> FAGGTVSQRCLSCICKMESGCRNVGCKMDMGSLSCGYFQIKEAYWIDCGRPGSSWKSCAASSYCASLCVQNYMKRYAKWAGCPLRCEGFARE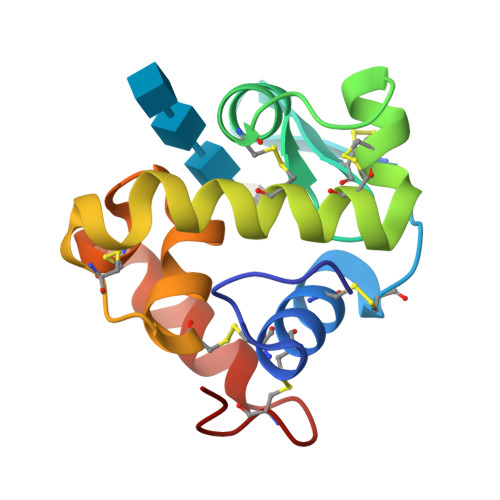HNGGPRGCKKGSTIGYWNRLQKISGCHGVQ1-benzothiophen-6-amine 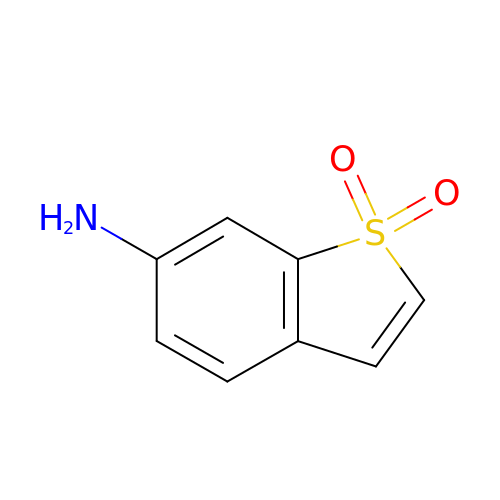1,1-dioxide | C8 H7 N O2 S | KRUCRVZSHWOMHC-UHFFFAOYSA-N>[3x]ASMTGGQQMGRGSASLPACPEESPLLVGPMLIEFNMPVDLELVAKQNPNVKMGGRYAPRDCVSPHKVAIIIPFRNRQEHLKYWLYYLHPVLQRQQLDYGIYVI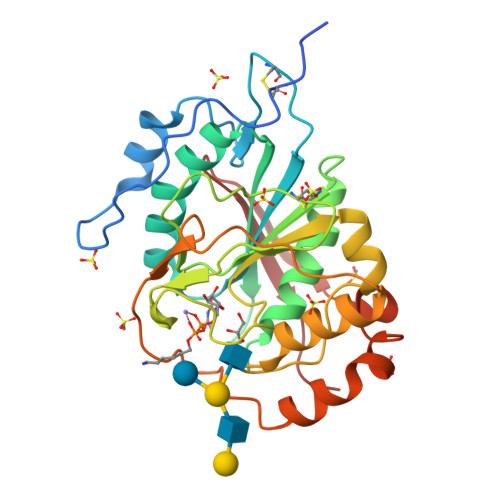NQAGDTIFNRAKLLNVGFQEALKDYDYTCFVFSDVDLIPMNDHNAYRCFSQPRHISVAMDKFGFSLPYVQYFGGVSALSKQQFLTINGFPNNYWGWGGEDDDIFNRLVFRGMSISRPNAVVGTTRHIRHSRDKKNEPNPQRFDRIAHTKETMLSDGLNSLTYQVLDVQRYPLYTQITVDIGTPS> QRRLYDQAKAALAKGNSAPYMASRSALRDYPLEPYLAYDELTHRLKSASNEEVERFLTEHGDLPQIGWLKLRWLRLLADRGDWKTFVNYYDPKLNFTELDCLYGQYQLGHGQK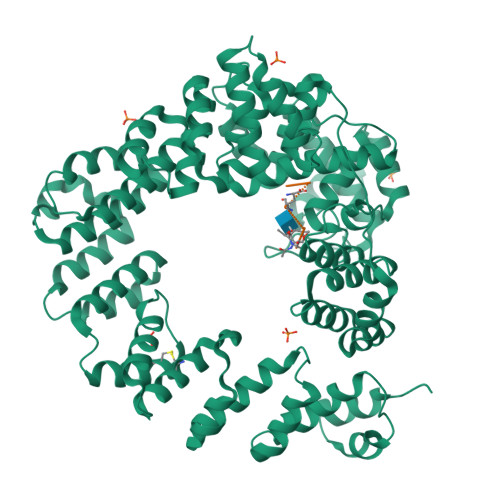AEGYATSERLWLVGKSQPAACDTLFGLWQGEGQLTEEKVWKRLKLAAEARNYSLASHLAQRLPTLGNQGALMVSVAQNPAQLSQTGRFSQRDHATADVVGLGLRRLARQDPEKALSLLDYYSSALPFSSDEKVAIAREIGLSLAKRFDPRALPLMTQYDPGLRDNTVTEWRTRLLLRLGRWDEAYALTRKLPQDLAATSRWRYWQARSLQLAQPNSKEPIALYQKLAGERDFYGFLAADRLSVPYKLGNRPAHIDPRVLQRVRNAASTRRAMEFFNRGEVINARREWYHAARLFDRDELIAQARLAYDMQWYFPAIRSISQAQYWDDLDIRFPMAHRATLVREAKNRGLHSSWIFAITRQESAFMSDARSGVGATGLMQLMPGTAKETSRKFGIPLASTQQLIVPDVNIRLGAAYLSQVHSQFNGNRVLASAAYNAGPGRVRQWLKDTRHLAFDVWIETIPFDETRQYVQNVLSYAVIYGQKLNAPQPIVDWHERYF;> AEKAA N-[1-HYDROXYCARBOXYETHYL-CARBONYL]LEUCYLAMINO-2-METHYL-BUTANE | C15 H28 N2 O5 | 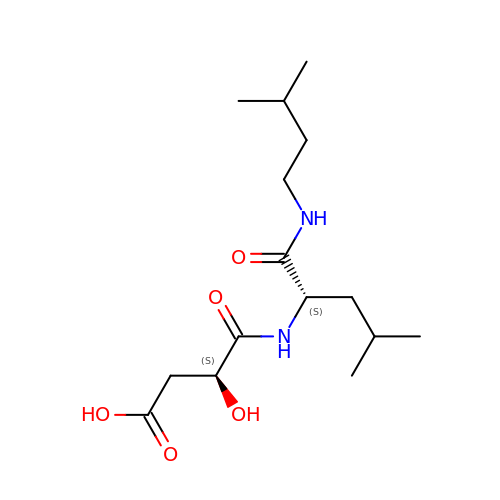KBIWEWPGBHKYML-RYUDHWBXSA-N> GEIEFIESSKDAGFPVINTPSKTKLEPSVFHQVFEGNKEPAVLRSGDPRLKANFEEAIFSKYIGNVNTHVDEYMLEAVDHYAGQLATLDISTEPMKLEDAVYGTEGLEALDLTTSAGYPYVALGIKKRDILSKKTKDLTKLKECMDKYGLNLPMVTYVKDELRSIEKVAKGKSRLIEASSLNDSVAMRQTFGNLYKTFHLNPGVVTGSAVGCDPDLFWSKIPVMLDGHLIAFDYSGYDASLSPVWFACLKMILEKLGYTHKETNYIDYLCNSHHLYRDKHYFVRGGMPSGCSGTSIFNSMINNIIIRTLMLKVYKGIDLDQFRMIAYGDDVIASYPWPIDGSLLAEAGKGYGLIMTPADKGECFNEVTWTNVTFLKRYFRADEQYPFLVHPVMPMKDI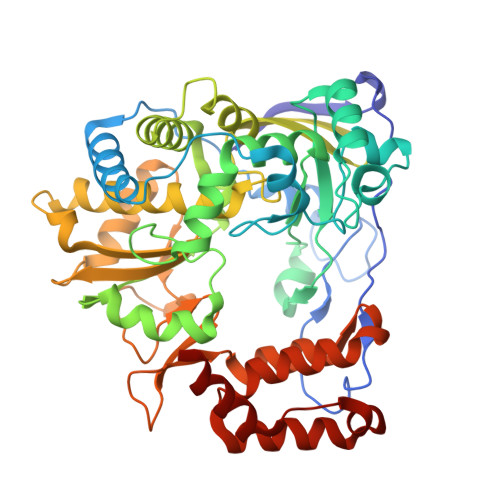HESIRWTKDPKNTQDHVRSLCLLAWHNGEHEYEEFIRKIRSVPVGRCLTLPAFSTLRRKWLDSF4-BROMO-3-(5'-CARBOXY-4'-CHLORO-2'-FLUOROPHENYL)-1-METHYL-5-TRIFLUOROMETHYL-PYRAZOL 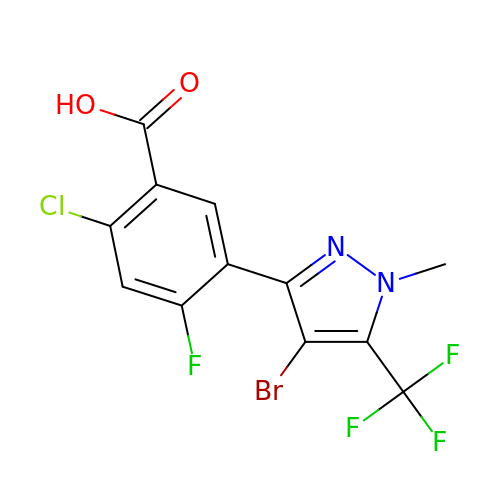| C12 H6 Br Cl F4 N2 O2 | YNMHKERYELPEEF-UHFFFAOYSA-N Clathrin-mediated endocytosis is essential for protein retrieval during neurotransmission and receptor recycling. Accumulation of the adapter proteins at the plasma membrane initiates the endocytic event and contributes to membrane bending. Complex formation has been observed between the ENTH domain of epsin and the ANTH domain of Sla2, the yeast homolog of human huntingtin interacting protein 1 related (Hip1R). Epsin and the phospholipid PIP2 are essential for clathrin-mediated endocytosis, and we show how assemblies are formed between the ENTH domain of epsin and the ANTH domain of Sla2 in fungi.

As a further indication that the ENTH2 dimer, which sandwiched PIP2, is functionally relevant, a similar dimer interface is observed in a crystal structure of the epsin Ent1 ENTH domain (ENTH1) from S. cerevisiae at 2.9 Å resolution. Here, a 2-methyl-2,4-pentanediol (MPD) molecule from the crystallization solution has caused a displacement of the α0 helix to allow dimer formation between ENTH1 domains. Native MS on a Thr104Glu mutant of ENTH1 from S. cerevisiae shows a reduction of PIP2 binding, where the binding of two PIP2 molecules is barely observed, indicating impairment of the binding site.

>[3x]MSKQFVRSAKNLVKGYSSTQVLVRNATSNDNHQVSKDSLIELAEKSYDSADFFEIMDMLDKRLNDKGKYWRHIAKALTVIDYLIRFGSENCVLWCRENLYIIKTLKEFRHEDDEGIDQGQIVRVKAKELTALLSDDERLNEERNMNIKGRNRKG>KHHHHHHIKPGALCVIDTPEGKGTGFFSGNDIVTAAHVVGNNTFVNVCYEGLMYEAKVRYMPEKDIAFITCPGDLHPTARLKLSKNPDYSCVTVMAYVNEDLVVSTAAAMVYGNTLSYAVRTQDGMSGAPVCDKYCRVLAVHQTNTGYTGGA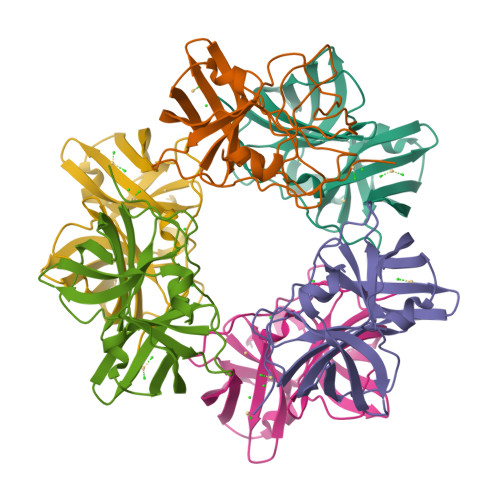VIIDPTDFHPV[6x]> SDTRKKRKDPDSDDWSESNSKENKID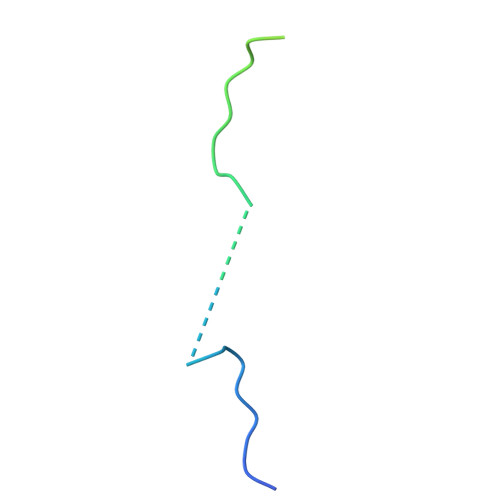NKHLNLLSSDSEIEQDYQKAKKRKTSDL> SDYMN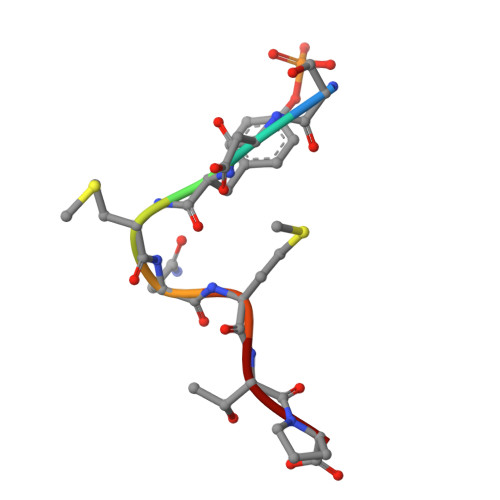MTP(2~{S},4~{S})-1-[(3~{S})-3-azanyl-3-(furan-2-yl)propanoyl]-4-cyclohexyl-~{N}-[(2~{S})-1-(methylamino)-1-oxidanylidene-3-pyridin-4-yl-propan-2-yl]pyrrolidine-2-carboxamide | C27 H37 N5 O4 | 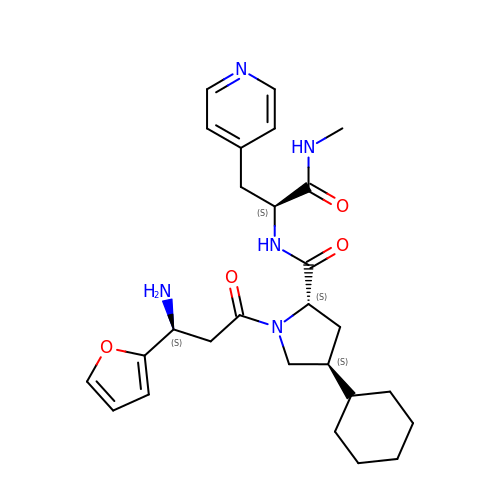SXOXGCGOYIMWNS-LDVJMBRRSA-N> MARYTMTLYDFIKSELIKKGFNEFVNDNKLTFYDDEFQFMQKMLKFDKDVLAIVNEKVFKGFSLKDELSDLLFKKSFTIHFLDREINRQTVEAFGMQVITVCITHEDYLNVVYSSSEVEKYLQSQ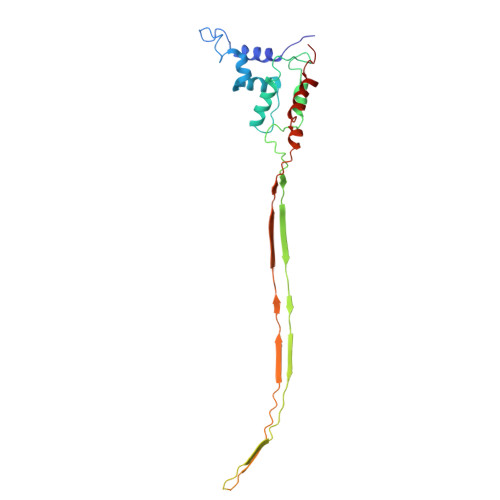GFTEHNEDTTSNTDETSNQNATSLDNSTGMTANRNAYVSLPQSEVNIDVDNTTLRFADNNTIDNGKTVNKSSNESNQNAKRNQNQKGNAKGTQFTKQYLIDNIDKAYDLRKKILNEFDKKCFLQIW>MTETPMMDDLERVLYNQDDIQKRIRELAAELTEFYEDKNPVMICVLTGAVFFYTDLLKHLDFQLEPDYIICSSYSGTKSTGNLTISKDLKTNIEGRHVLVVEDIIDTGLTMYQLLNNLQMRKPASLKVCTLCDKDIGKKAYDVPIDYCGFVVENRYIIGYGFDFHNKYRNLPVIGILKESVYT[2x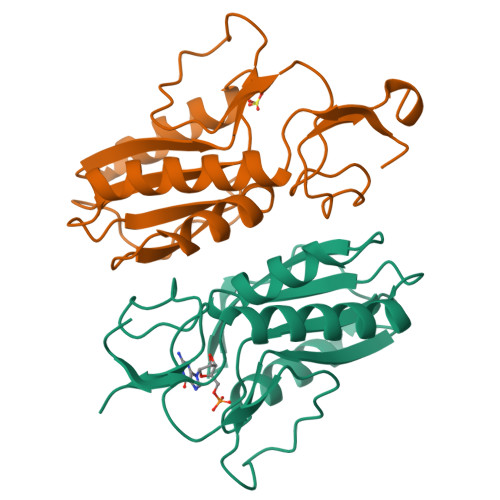]>SNAMEIIPIPADSYTLGFIGAGKMAESIAKGAVRSGVLSPSRIKTAIHSNPARRTAFESIGITVLSSNDDVVRDSNVVVFSVKPQLLKDVVLKLKPLLTKDKLLVSVAAGIKMKDLQEWAGHERFIRVMPNTAATVGEAASVMSLGGAATEEDANLISQLFGSIGKIWKADDKYFDAITGLSGSGPAYIYLAIEALADGGVAAGLPRDLALSLASQTVLGAASMATQSGKHPGQLKDDVTSPGGTTIAGVHELEKAGFRGILMNAVVAAAKRSQELS[10x]

The pathway preference appears to depend on nitrogen availability, being the ornithine route preferred under nitrogen-rich conditions. Both routes converge at the generation of P5C, which in the final step is reduced to L-proline by P5C reductase (P5CR, EC 1.5.1.2). Here we report the high-resolution crystal structure of P5CR from M. truncatula (Mt), a model legume plant. The donut-shaped decamer of MtP5CR can be described as a pentamer of symmetric, bean-like dimers that are related to each other by a five-fold NCS axis. The catalytic centers of P5CRs are located between the dinucleotide-binding domain (N-terminal) and the dimerization domain (C-terminal).

Concerning hydride donors, the complexes with NAD+ and NADP+ showed that both coenzymes are bound by the N-terminal domain of MtP5CR via multiple hydrogen bonds created mostly by the backbone N and O atoms of the protein. In the case of NAD+, the adenine N1 atom interacts with Nδ of Asn65. The N3 atom of adenine forms water-mediated hydrogen bonds with the backbone N and O of Ala18 and Ala43, respectively. Additionally, adenine interacts by π–stacking to His45 with an interplanar distance of about 3.6 Å and an inclination below 6°. The O atoms of the pyrophosphate group form strong ionic hydrogen bonds to the peptide amides of Lys20, Met21 and, via H2O, to Gly19 and Ala22. The nicotinamide-adjacent ribose forms two direct hydrogen bonds between O2′ and the backbone NH of Ala106, as well as between O3′ and the carbonyl of Val79. The si-side of the C4 carbon atom of the nicotinamide faces toward the catalytic center. This means that during the reduction reaction, the hydride would be transferred from the pro-S position of NAD(P)H. In the catalytic center of the enzyme, a MOPS molecule was also found in the structures with either coenzyme. NAD+ did not exert any inhibitory effect regardless of the coenzyme used.>[12x]DPEFGAGGPWEMRERLGTGGFGNVCLYQHRELDLKIAIKSCRLELSTKNRERWCHEIQIMKKLNHANVVKACDVPEELNILIHDVPLLAMEYCSGGDLRKLLNKPENCCGLKESQILSLLSDIGSGIRYLHENKIIHRDLKPENIVLQDVGGKIIHKIIDLGYAKDVDQGELCTEFVGTLQYLAPELFENKPYTATVDYWSFGTMVFECIAGYRPFLHHLQPFTWHEKIKKKDPKCIFACEEMSGEVRFSSHLPQPNSLCSLIVEPMENWLQLMLNWDPQQRGGPVDLTLKQPRCFVLMDHILNLKIVHILNMTSAKIISFLLPPDESLHSLQSRIERETGINTGSQELLSETGISLDPRKPASQCVLDGVRGCDSYMVYLFDKSKTVYEGPFASRSLSDCVNYIVQDSKIQLPIIQLRKVWAEAVHYVSGLKEDYSRLFQGQRAAMLSLLRYNANL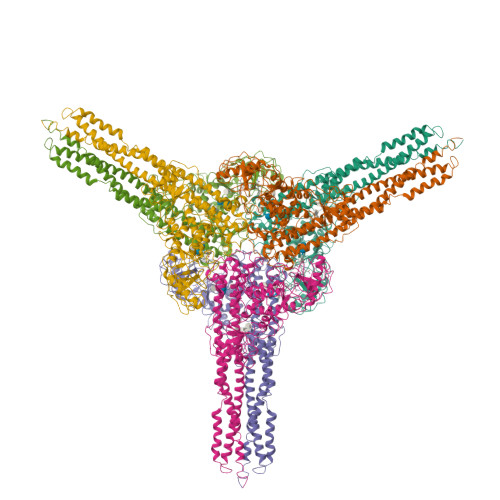TKMKNTLISASQQLKAKLEFFHKSIQLDLERYSEQMTYGISSEKMLKAWKEMEEKAIHYAEVGVIGYLEDQIMSLHAEIMELQKSPYGRRQGDLMESLEQRAIDLYKQLKHRPSDHSYSDSTEMVKIIVHTVQSQDRVLKELFGHLSKLLGCKQKIIDLLPKVEVALSNIKEADNTVMFMQGKRQKEIWHLLKIACTQ>GQDIQLIPPLINLLMSIEPDVIYAGHDNTKPDTSSSLLTSLNQLGERQLLSVVKWSKSLPGFRNLHIDDQITLIQYSWMSLMVFGLGWRSYKHVSGQMLYFAPDLILNEQRMKE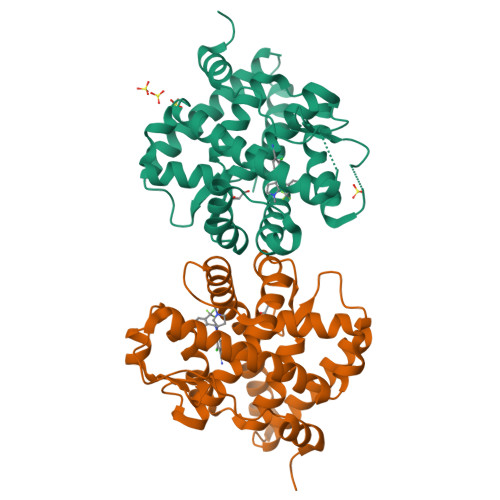SSFYSLCLTMWQIPQEFVKLQVSQEEFLCMKVLLLLNTIPLEGLRSQTQFEEMRSSYIRELIKAIGLRQKGVVSSSQRFYQLTKLLDNLHDLVKQLHLYCLNTFIQSRALSVEFPEMMSEVIAAQLPKILAGMVKPLLFHKK[2x]>MARPKSEDKKQALLEAATQAIAQSGIAASTAVIARNAGVAEGTLFRYFATKDELINTLYLHLRQDLCQSLIMELDRSITDAKMMMRFIWNSGISWGLNHPARHRAIRQLAVSEKLTKETHQRDLDMFPELRDILHRRVLMVFMSDEYRAFGDGLFLALAETTMDFAARDPARAGEYIALGF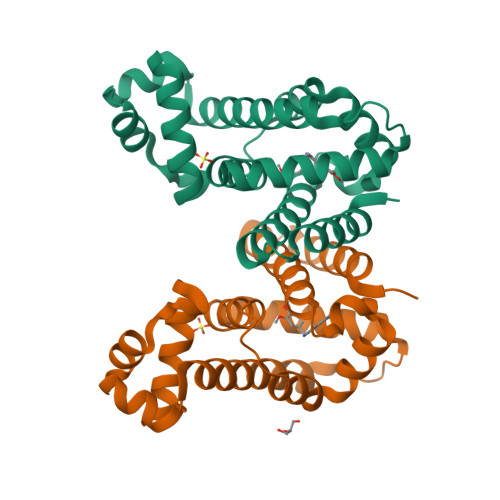EAMWRALTREEQ[2x]>[4x]MNETSHEASECPAAVITGGARRIGHSIAVRLHQQGFRVVVHYRHSEGAAQRLVAELNAARAGSAVLCKGDLSLSSSLLDCCEDIIDCSFRAFGRCDVLVNNASAYYPTPLLPGDDTNGAADAKPIDAQVAELFGSNAVAPLFLIRAFARRQGEGGAWRSRNLSVVNLCDAMTDLPLPGFCVYTMAKHALG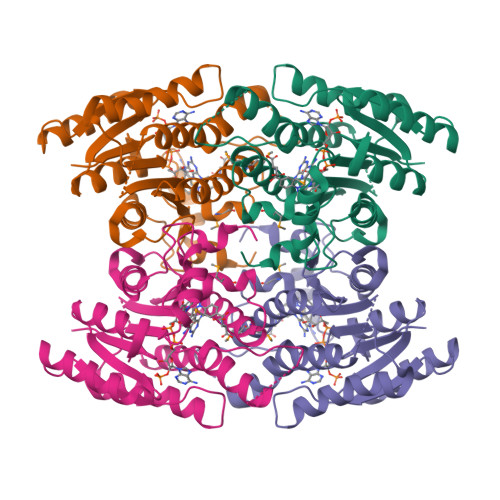GLTRAAALELAPRHIRVNAVAPGLSLLPPAMPQETQEEYRRKVPLGQSEASAAQIADAIAFLVSKDAGYITGTTLKVDGGLILARA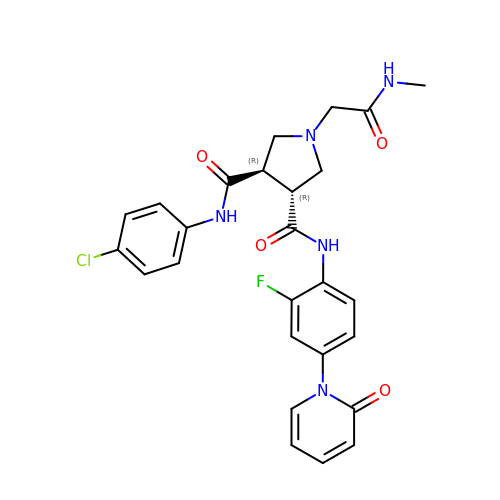(3R,4R)-1-METHYLCARBAMOYLMETHYL-PYRROLIDINE-3,4-DICARBOXYLIC ACID 3-[(4-CHLORO-PHENYL)-AMIDE] 4-{[2-FLUORO-4-(2-OXO-2H-PYRIDIN-1-YL)-PHENYL]-AMIDE} | C26 H25 Cl F N5 O4 | DXHIEYAKKGEXDY-PMACEKPBSA-N> GSMVVIANAHNELIHDAVLDYYGKRLATCSSDKTIKIFEVEGETHKLIDTLTGHEGPVWRVDWAHPKFGTILASCSYDGKVLIWKEENGRWSQIAVHAVHSASVNSVQWAPHEYGPLLLVASSDGKVSVVEFKENGTTSPIIIDAHAIGVNSASWAPATIEEDGEHNGTKESRKFVTGGADNLVKIWKYNSDAQTYVLESTLEGHSDWVRDVAWSPTVLLRSYLASVSQDRTCIIWTQDNEQGPWKKTLL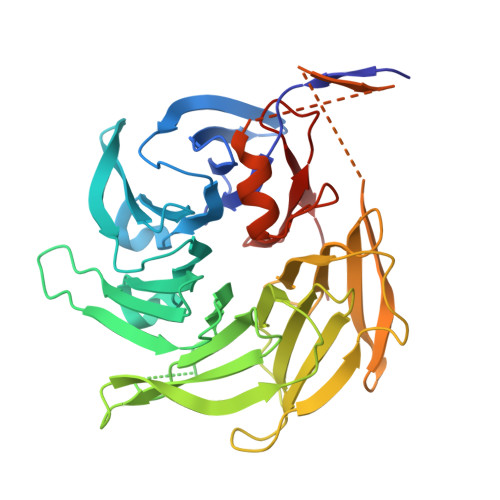KEEKFPDVLWRASWSLSGNVLALSGGDNKVTLWKENLEGKWEPAGEVHQGGGGSGGGGATSKEFDGPCQNEIDLLFSECNDEIDNAKLIMKERRFTASYTFAKFSTGSMLLTKDIVGKSGVSIKRLPTE> PISPIETVPVKLKPGMDGPKVKQWPLTEEKIKALVEICTEMEKEGKISKIGPENPYNTPVFAIKKKDSTKWRKLVDFRELNKRTQDFWEVQLGIPHPAGLKKKKSVTVLDVGDAYFSVPLDEDFRKYTAFTIPSINNETPGIRYQYNVLPQGWKGSPAIFQSSMTKILEPFKKQNPDIVIYQYMDDLYVGSDLEIGQHRTKIEELRQHLLRWGLTTPDKKHQKEPPFLWMGYELHPDKWTVQPIVLPEKDSWTVNDICKLVGKLNWASQIYPGIKVRQLSKLLRGTKALTEVIPLTEEAELELAENREILKEPVHGVYYDPSKDLIAEIQKQGQGQWTYQIYQEPFKNLKTGKYARMRGAHTNDVKQLTEAVQKITTESIVIWGKTPKFKLPIQKETWETWWTEYWQATWIPEWEFVNTPPLVKLWYQLEKEPIVGAETFYVDGAANRETKLGKAGYVTNKGRQKVVPLTNTTNQKTELQAIYLALQDSGLEVNIVTDSQYALGIIQAQPDKSESELVNQIIEQLIKKEKVYLAWVPAHKGIGGNEQVDKLVSAGIRK;> PISPIETVPVKLKPGMDGPKVKQWPLTEEKIKALVEICTEMEKEGKISKIGPENPYNTPVFAIKKKDSTKWRKLVDFRELNKRTQDFWEVQLGIPHPAGLKKKKSVTVLDVGDAYFSVPLDEDFRKYTAFTIPSINNETPGIRYQYNVLPQGWKGSPAIFQSSMTKILEPFRKQNPDIVIYQYMDDLYVGSDLEIGQHRTKIEELRQHLLRWGLTTPDKKHQKEPPFLWMGYELHPDKWTVQPIVLPEKDSWTVNDIQKLVGKLNWASQIYPGIKVRQLSKLLRG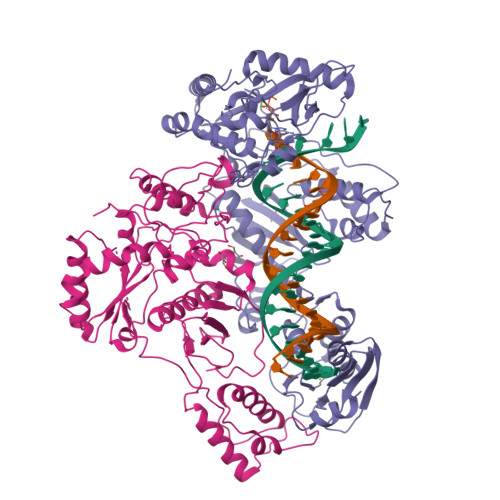TKALTEVIPLTEEAELELAENREILKEPVHGVYYDPSKDLIAEIQKQGQGQWTYQIYQEPFKNLKTGKYARMRGAHTNDVKQLTEAVQKITTESIVIWGKTPKFKLPIQKETWETWWTEYWQATWIPEWEFVNTPPLVKLWYQLGGHHHHHH The global gene regulator known as regulator of proteinase B (RopB) and an eight amino acid leaderless peptide signal, SpeB-inducing peptide (SIP), form an intracellular receptor and intercellular peptide signal pair that controls speB expression. The SIP peptide is produced and secreted during high-bacterial population density and reimported into the bacterial cytosol, where it directly interacts with cytosolic RopB37. SIP promotes high-affinity RopB-speB promoter interactions and RopB oligomerization. GAS integrates a pH-sensing mechanism with the SIP signaling pathway through a pH-sensitive histidine switch in RopB.

Thus, to help elucidate the molecular basis for pH dependent, and sequence-specific SIP recognition by RopB, we crystallized the C-terminal domain of RopB (RopB–CTD) bound to SIP. Thus, we used RopB–CTD that has the entire tetratricopeptide repeat (TPR) domain (amino acids 56–280) containing the putative peptide-binding pocket but lacks the N-terminal DNA-binding domain (amino acids 1–55). Thus, the region containing amino acids 159–200 of RopB was built as single α helix in the RopB–CTD–SIP structure. Each asymmetric unit has two subunits of RopB–CTD, and only one subunit in the asymmetric unit has defined electron density for SIP. SIP is oriented with its N-terminus facing the solvent-exposed exterior of the pocket, whereas the C-terminus is buried in the deep end of the pocket. The SIP-binding surface in RopB is formed by helix α6 of TPR 3, helix α8 of TPR 4, and the C-terminal capping helix α12. The peptide-contacting face of helix α6 is lined by N152 and F155, and the surface of helix α8 facing SIP has R188, N192, I195, and Q199. The side chains of M267, F268, Y271, and K278 of the capping helix α12 are positioned to interact with SIP. Given that RopB–CTD has decreased affinity for SIP compared to full-length RopB, and RopB–CTD–SIP was crystallized under nonoptimal pH (pH 7.5) for RopB–SIP interactions, it is likely that the structure of RopB–CTD–SIP represents a low-affinity state. In the structure of RopB–CTD crystallized at pH 7.5, the side chains of Y182’ and E185’ (where ‘ indicates the amino acids from the second subunit of a RopB–CTD dimer) are oriented toward H144 but located farther (5.8 and 4.9 Å, respectively) to interact with H144.

>[2x]NVDEFLFISNNFKQYKEFIDMDTAKHYFECRNIEGLNHILDSYKDSKSTKEKNLFALVKVLLATLTEEDCLTERTYLSNYLINIETWSHYETVLFNNCMFIFESCFIEMVFSKVILNLDKYNTLRYYGNESIRMFVNMLILFIQRQEYDKASEILAKIEDYQLNDDCLYERCCVSFFDGIIGLINGKEGAEQKCVQILEIFQLLNCKTIHHMFQTYLEAIKHKLSLEHHHHHH;> MWLLLLFL> AAAMKLAYWMYAGPAHIGTLRIASSF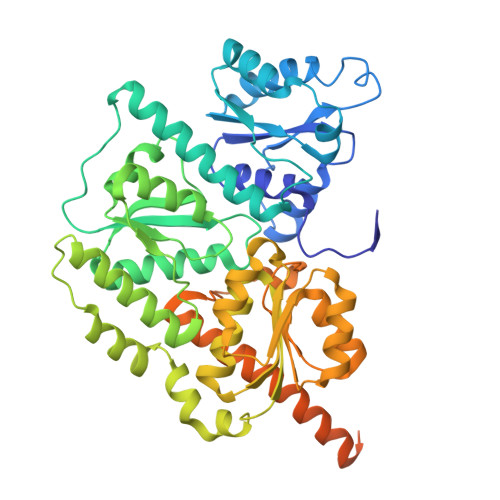KNVHGIMHAPLGDDYFNVMRSMLERERDFTPVTASIVDRHVLARGSQEKVVDNIIRKDTEEHPDLIVLTPTCTSSILQEDLQNFVRRASLSTTADVLLADVNHYRVNELQAADRTLEQIVQFYIDKARRQGTLGTSKTPTPSVNIIGITTLGFHNQHDCRELKQLMADLGIQVNLVIPAAATVHDLQRLPQAWFNLVPYREIGGLTAQYLEREFGQPSVRITPMGVVETARCIRAIQGVLNAQGAGVNYEAFIEQQTREVSQAAWFSRSIDCQNLTGKKAVVFGDNTHAAAMTKILSREMGIHVVWAGTYCKYDADWFRAEVAGFCDEVLITDDHTVVGDAIARVEPAAIFGTQMERHVGKRLNIPCGVIAAPIHIQDFPVGYRPFLGYEGTNQLVDLIYNSFTLGMEDHLLEIFGGHDTKAVIHKGLSADSDLTWTAAGLAELNKIPGFVRGKVKRNTEKFAREQGISEITVEVLYAAKEAVGA> MEGSTGFDGDATTFFAPDAVFGDRVRRFQEFLDTFTSYRDSVRSIQVYNSNNAANYNDDQDDADERDLLGDDDGDDLEKEKKAASSTSLNILPHRIIISLDDLREFDRSFWSGILVEPAYFIPPAEKALTDLADSMDDVPHPNASAVSSRHPWKLSFKGSFGAHALSPRTLTAQHLNKLVSVEGIVTKTSLVRPKLIRSVHYAAKTGRFHYRDYTDATTTLTTRIPTPAIYPTEDTEGNKLTTEYGYSTFIDHQRITVQEMPEMAPAGQLPRSIDVILDDDLVDKTKPGDRVNVVGVFKSLGAGGMNQSNSNTLIGFKTLILGNTVYPLHARSTGVAARQMLTDFDIRNINKLSKKKDIFDILSQSLAPSIYGHDHIKKAILLMLMGGVEKNLENGSHLRGDINILMVGDPSTAKSQLLRFVLNTASLAIATTGRGSSGVGLTAAVTTDRETGERRLEAGAMVLADRGVVC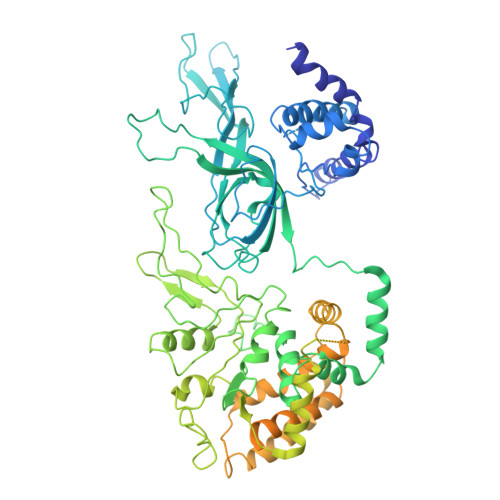IDEFDKMTDVDRVAIHEVMEQQTVTIAKAGIHTTLNARCSVIAAANPVFGQYDVNRDPHQNIALPDSLLSRFDLLFVVTDDINEIRDRSISEHVLRTHRYLPPGYLEGEPVRERLNLSLAVGEDADINPEEHSNSGAGVENEGEDDEDHVFEKFNPLLQAGAKLAKNKGNYNGTEIPKLVTIPFLRKYVQYAKERVIPQLTQEAINVIVKNYTDLRNDDNTKKSPITARTLETLIRLATAHAKVRLSKTVNKVDAKVAANLLRFALLGEDIGNDIDEEESEYEEALSKRSPQKSPKKRQRVRQPASNSGSPIKSTPRRSTASSVNATPSSARRILRFQDDEQNAGEDDNDIMSPLPADEEAELQRRLQLGLRVSPRRREHLHAPEEGSSGPLTEVGTPRLPNVSSAGQDDEQQQSVISFDNVEPGTISTGRLSLISGIIARLMQTEIFEEESYPVASLFERINEELPEEEKFSAQEYLAGLKIMSDRNNLMVADDKVWRV>MATNNNQIGENKEQTIFDHKGNVIKTEDREIQIISKFEEPLIVVLGNVLSDEECDELIELSKSKLARSKVGSSRDVNDIRTSSGAFLDDNELTAKIEKRISSIMNVPASHGEGLHILNYEVDQQYKAHYDYFAEHSRSAANNRISTLVMYLNDVEEGGETFFPKLNLSVHPRKGMAVYFEYFYQ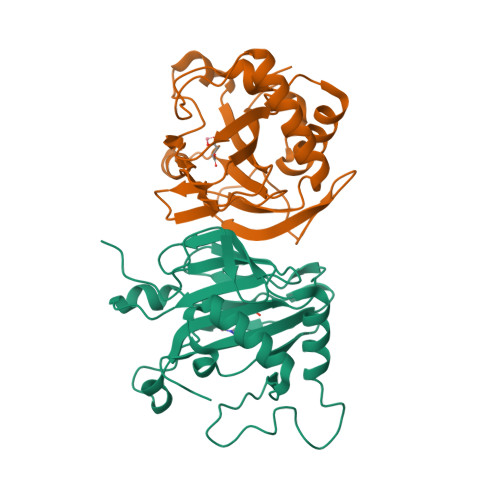DQSLNELTLHGGAPVTKGEKWIATQWVRRGTYK[4x]However, we were successful in performing structural study of a newly discovered bacterial RNA repair complex consisting of three proteins named Pnkp1, Rnl and Hen1, which form a heterohexamer in vitro. Since the newly found RNA repair system possesses elements of both T4 and Pnkp–Hen1 RNA repair systems, it can be regarded as a hybrid RNA repair system. Therefore, the Pnkp1–Rnl–Hen1 heterohexamer is likely the functional unit of a new bacterial RNA repair system in vivo. Because the Pnkp1–Rnl–Hen1 RNA heterohexamer possesses two identical copies of each enzymatic activity, a total of eight active sites are present in the complex, same as in the RNA repair complex of the Pnkp–Hen1 heterotetramer.

We crystallized the Pnkp1–Rnl–Hen1 heterohexamer and solved the structure at 3.3 Å resolution. The structure confirmed several observations from the chromatographic experiments, including the formation of Pnkp1 homodimer, Pnkp1–Rnl interaction and Rnl–Hen1 interaction. Unexpectedly, Pnkp1 and Hen1 were found to make physical contact in the structure, which was not the case with the chromatographic analysis. As a result of the additional Pnkp1–Hen1 interaction, each protein makes physical contacts with the other two proteins, resulting in the Pnkp1–Rnl–Hen1 heterotrimer adopting a ring structure. Because Pnkp1 forms a homodimer (coloured cyan and sand), the overall architecture of the Pnkp1–Rnl–Hen1 heterohexamer consists of two rhomboid-shaped ring structures of Pnkp1–Rnl–Hen1 heterotrimers fused at the Pnkp1 dimer interface. The side view of the structure displays C2 symmetry, suggesting the presence of two functional units of the RNA repair machinery having RNA substrates approach from opposite directions (indicated by arrows). On the local level, the Pnkp1 homodimer is formed by interactions between the same enzymatic domains, resulting in kinase and phosphatase dimer modules. In the structure of the Pnkp1–Rnl–Hen1 heterohexamer, however, the relative orientation of the kinase and phosphatase modules is locked at 130°. For the Pnkp1–Rnl interaction, each copy of Rnl makes contact with a single copy of Pnkp1 at the kinase domain. On the other hand, each copy of Hen1 make contacts with both copies of Pnkp1.

>MSAKNNTHHFPKLLILVGAPGSGKSTFARYFIRTEDNWVRVNRDDFRLMQFGDSLMSPFYEERITKMVEASVIALLKNRTNVIIDATNSSLRSLQDMVHTYTEYADISFKVFDLPVEELVKRCDKRCEQTGKFIPKSAIEKHVTQLQYTKEKFDFKPIPRALKETSLTYADQDTSLPKAVICDLDGTLSLLNGRDPYNASTADQDLLNTPVAMVLKMAKQQGYKVILLSGRENAYREPTERFLAKYQIDYDLLLMRDTNDYRKDNIIKKELFLEEIQGKYFVEFLLDDRNQVVDMWRRELALPCFQVNYGDF[2x];>MEDKTLIKKRIDWFCKNKINAFSPTISPAPKSVERNEIESLYEGILWFVLNGVKEIVIEKKYMGSYCDIYLHRRLEDTYLVSRNGYKINHLDQEQCLRALQGLHDRFSWDGVELRIIQSELMPWSILGKGLINNEFSAYYISHEIHAEYLVQSSLYEKLQKIQQEPAYLSFVADAKVLSAKELKDKYPMHIIRQYQSIRDFKFLDLPHYQQNIQLFKRQLDIFGKEAAPFFKPFNILKEVYTDGREHFVNDNLSFQQINDDDFLHYQFADREDFEAKYPQIRAWVDQVNQSDEEGVVIKPRTAFLPGMPPAFKVRNNDYLTLVYGVDFQDRLQEQIAKRNIKGKLRCSINDWAINAKLLAIPYSELGEENYELKNLVLDRILGEEIENQLDSRL[2x];>[2x]MILQIHSQNPHLLDLLNKNPHTDLGIYAKSLRNGQLIGNAVSAYQYDVVFQDTRYSYLPEESNQIDFQSYCSPLVILHICNEFFKELLQEKQTYWSQQIKWLERTRAEVDTYPCTIEVKNLYANSTWYSKGHFMMERYFKNIHITPIVGNNLSLRVEGKSVFEAMNLLSFIAVTTHITNTYGEYTYIDDHFAQKYARILTNIPQVPYFVFYLFIKRAIKSERQFAEIKPMFEAYFKEEGLDIDFQFTDTHGSRMDFIVKELGMEYPILDIGCGELKYYRRFMRRNYNYSHPYFATDTDKSVGDYAALLKERMEADNLYFFSDWTDYEYKNPVNIILTEVIEHNTPEAAEALVKHCLSLNFHKMIITTPNSLFNKYYFDEDPESLRHEDHHFEWTPQEFQDFIRHCVGDTSLEVTYCGIGDRINGETPTQAVVITRK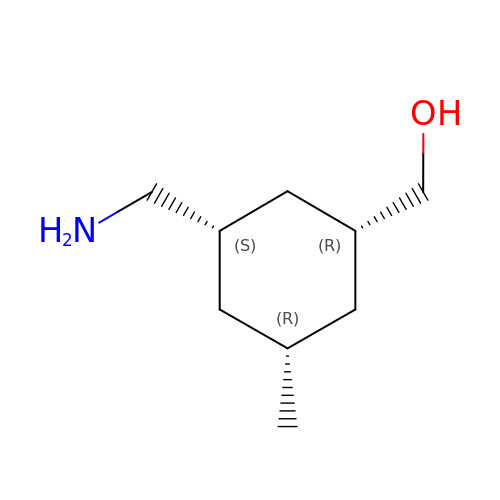[(1R,3S,5R)-3-(aminomethyl)-5-methyl-cyclohexyl]methanol | C9 H19 N O | OCRWQOBBCGSFAT-HRDYMLBCSA-N>[2x]GSMKLFAQGTSLDLSHPHVMGILNVTPDSFSDGGTHNSLIDAVKHANLMINAGATIIDVGGESTRPGAAEVSVEEELQRVIPVVEAIAQRFEVWISVDTSKPEVIRESAKVGAHIINDIRSLSEPGALEAAAETGLPVCLMHMQGNPKTMQEAPKYDDVFAEVNRYFIEQIARCEQAGIAKEKLLLDPG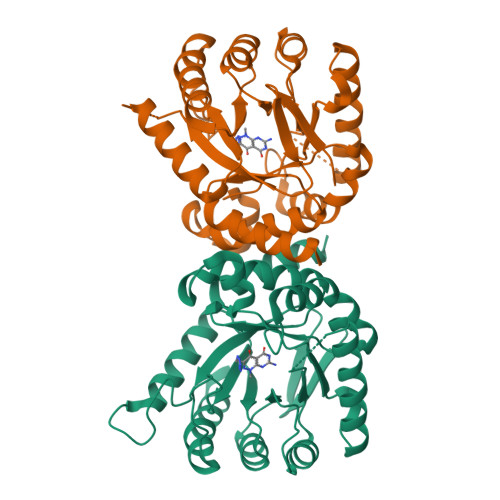FGFGKNLSHNYSLLARLAEFHHFNLPLLVGMSRKSMIGQLLNVGPSERLSGSLACAVIAAMQGAHIIRVHDVKETVEAMRVVEATLSA>GGCUAGCUGGAGGGGCGCCAGUUCGCUGGUGGUUGGG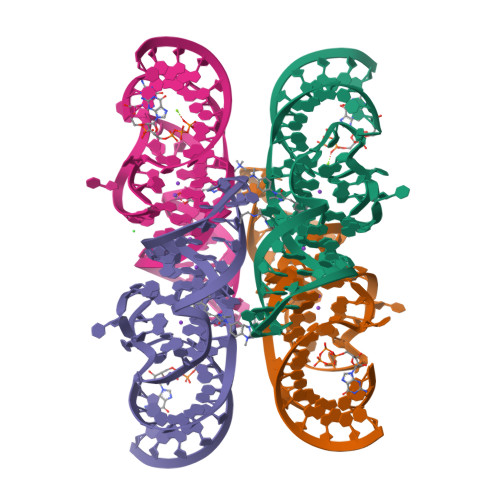UGCGGUCGGCUAGCC[4x]> GSGKFGQQSGAIYVGNFRVVNRHLATHNDWANLVWEDSSRDLLVSSTTAQGCDTIARCNCQTGVYYCNSRRKHYPVSFSKPSLIYVEASEYYPARYQSHLMLAQGHSEPGDAGGILRCQHGVVGIVSTGGN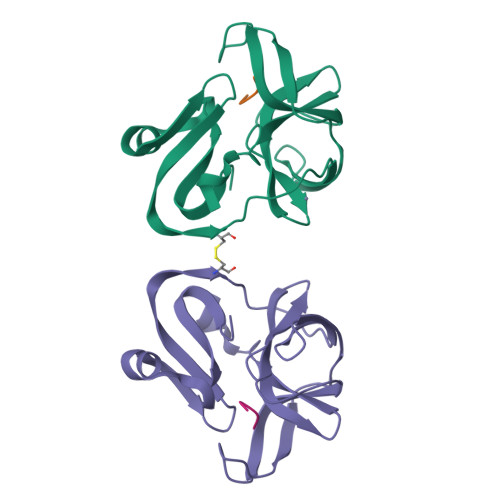GLVGFADVRDLLWLDEEAMEQ;> GSITTLGKFG> MHHHHHHHHHHSGQNLYFQGHMATFISVQLKKTSEVDLAKPLVKFIQQTYPSGGEEQAQYCRAAEELSKLRRAAVGRPLDKHEGALETLLRYYDQICSIEPKFPFSENQICLTFTWKDAFDKGSLFGGSVKLALASLGYEKSCVLFNCAALASQIAAEQNLDNDEGLKIAAKHYQFASGAFLHIKETVLSALSREPTVDISPDTVGTLSLIMLAQAQEVFFLKATRDKMK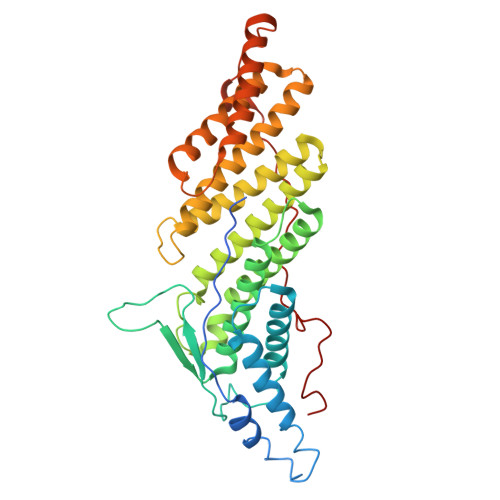DAIIAKLANQAADYFGDAFKQCQYKDTLPKEVFPVLAAKHCIMQANAEYHQSILAKQQKKFGEEIARLQHAAELIKTVASRYDEYVNVKDFSDKINRALAAAKKDNDFIYHDRVPDLKDLDPIGKATLVKSTPVNVPISQKFTDLFEKMV>VIPPISCPENEKGPFPKNLVQIKSNKDKEGKVFYSITGQGADTPPVGVFIIERETGWLKVTEPLDR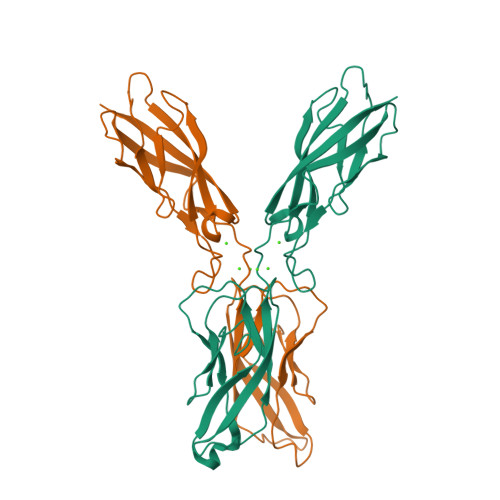ERIATYTLFSHAVSSNGNAVEDPMEILITVTDQNDNKPEFTQEVFKGSVMEGALPGTSVMEVTATDADDDVNTYNAAIAYTILSQDPELPDKNMFTINRNTGVISVVTTGLDRESFPTYTLVVQAADLQGEGLSTTATAVITVTD[2x]>MTYVILPLEMKKGRGYVYQLEYHLIWCVKYRHQVLVGEVADGLKDILRDIAAQNGLEVITMEVMPDHVHLLLSATPQQAIPDFVKALKGASARRMFVAYPQLKEKLWGGNLWNPSYCILTVSENTRAQIQKYIESQHD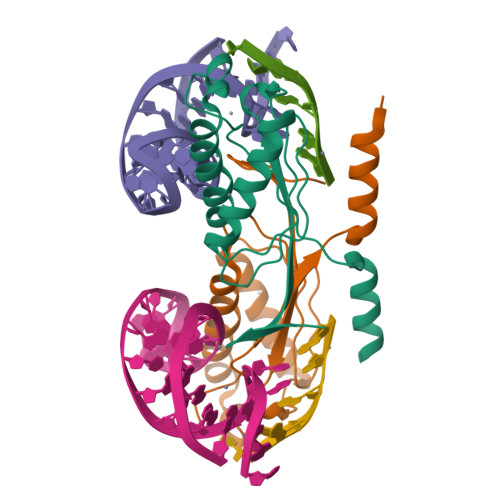KE[2x]>CGIVGIAGVMPVNQSIYDALTVLQHRGQDAAGIITIDANNCFRLRKANGLVSDVFEARHMQRLQGNMGIGHVRYPTAGSSSASEAQPFYVNSPYGITLAHNGNLTNAHELRKKLFEEKRRHINTTSDSEILLNIFASELDNFRHYPLEADNIFAAIAATNRLIRGAYACVAMIIGHGMVAFRDPNGIRPLVLGKRDIDENRTEYMVASESVALDTLGFDFLRDVAPGEAIYITEEGQLFTRQCADNPVSNPCLFEYVYFARPDSFIDKISVYSARVNMGTKLGEKIAREWEDLDIDVVIPIPETSCDIALEIARILGKPYRQGFVKNRYVGRTFIMPGQQLRRKSVRRKLNANRAEFRDKNVLLVDDSIVRGTTSEQIIEMAREAGAKKVYLASAAPEIRFPNVY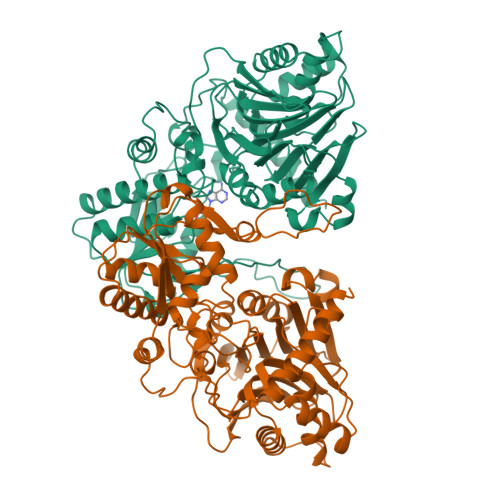GIDMPSATELIAHGREVDEIRQIIGADGLIFQDLNDLIDAVRAENPDIQQFECSVFNGVYVTKDVDQGYLDFLDTLRNDDAKAVQRQNEVENLEMHNEG[4x]3-azanyl-3-azanylidene-propanamide | C3 H7 N3 O | 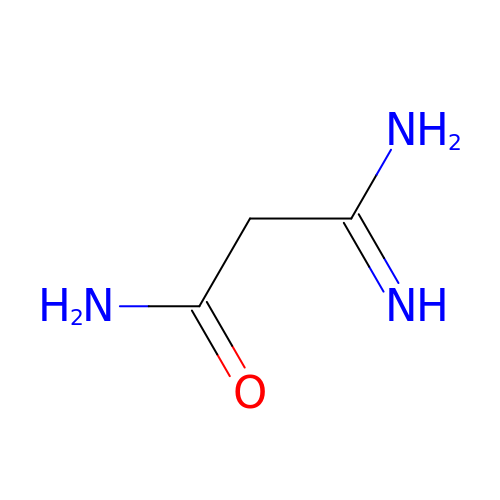RGXJMLZFKIUGNH-UHFFFAOYSA-N(1R,3S,5Z)-5-[(2E)-2-[(1R,3aS,7aR)-1-[(E,2R,5S)-5,6-dimethyl-6-oxidanyl-hept-3-en-2-yl]-7a-methyl-2,3,3a,5,6,7-hexahydro-1H-inden-4-ylidene]ethylidene]-4-methylidene-cyclohexane-1,3-diol 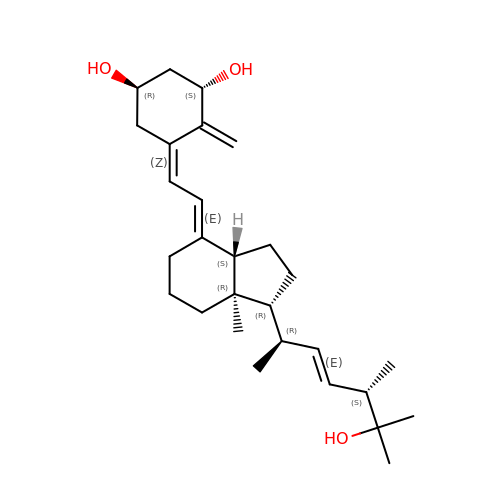| C28 H44 O3 | ZGLHBRQAEXKACO-XJRQOBMKSA-N>GPMSTIGATHNVRVVGSGRKTIVLGNGYGTDQSVWRHLVPHLVGRYKVLLYDNMGAGTTNPDYYDFDRYATLEGFAYDLLAILEEFNVRKCIYVGHSMAAMVGMIASIFRPDLFHKLITISATPRMSNTDDYYGGFEQEELDQMDEGLRMNHESMIRGMAPLVVGGDMDSEAVHEYTRMLLNMRPDIALSLSRTLYAFDMRPFLGQVTVPCH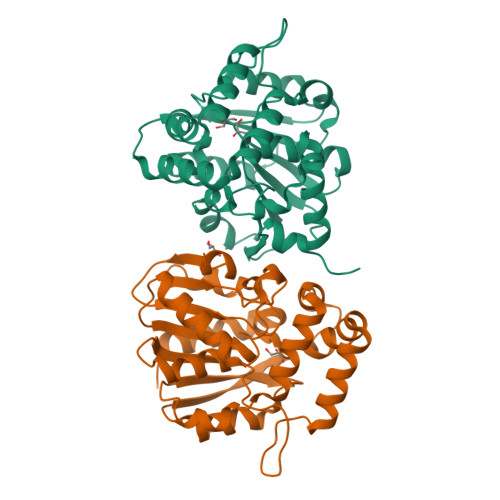ILQSSKDMGVPVAVAEYLHQSLGGKSIVEVMSAEGHLPHLSAPEITIPVLLRHIQQDI[2x]>[2x]GPDMNNELHNENTIRILISSDPHVGYGEKDPVRGNDSFVSFNEILEIARERDVDMILLGGDIFHDNKPSRKALYQALRSLRLNCLGDKPCELELLSDTSLTTGDTAVCNINYLDPNINVAIPVFSIHGNHDDPSGDGRYSALDILQVTGLVNYF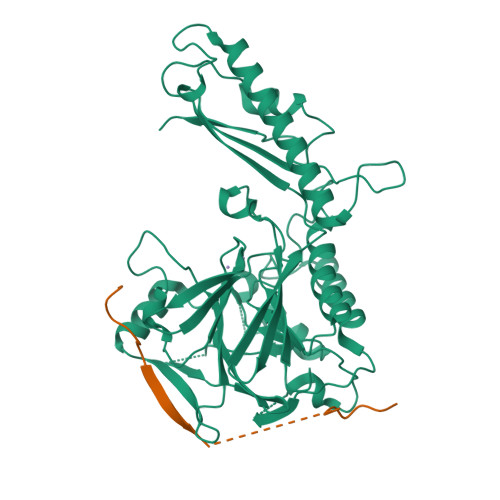GRVPENDNIVVSPILLQKGFTKLALYGISNVRDERLYHSFRENKVKFLRPDLYRDEWFNLLTVHQNHSAHTPTSYLPESFIQDFYDFVLWGHEHECLIDGSYNPTQKFTVVQPGSTIATSLSPGETAPKHCGILNITGKDFHLEKIRLRTVRPFIMKDIILSEVSSIPPMVENKKEVLTYLISKVEEAITEANAQWYEAQGTVPVVENEKPPLPLIRLRVDYTGGYQTENPQRFSNRFVGRVANATDVVQFYLKKVDENLYFQ;>GESEDDKAFEENRRLRNLGSVEYIRIMSSEKSNANSRHTSKYYSGRKNFKKFQKKASQK[2x]>RAPAPATPHAPDHSPAPNSPTLTRPPEGPKFPRVKNWELGSITYDTLCAQSQQDGPCTPRRCLGSLVLPRKLQTRPSPGPPPAEQLLSQARDFINQYYSSIKRSGSQAHEERLQEVEAEVASTGTYHLRESELVFGAKQAWRNAPRCVGRIQWGKLQVFDARDCSSAQEMFTYICNHIKYATNRGNLRSAITVFPQRAPGRGDFRIWNSQLVRYAGYRQQDGSVRGDPANVEITELCIQHGWTPGNGRFDVLPLLLQAPDEAPELFVLPPELVLEVPLEHPTLEWFAALGLRWYALPAVSNMLLEIGGLEFSAAPFSGWYMSTEIGTRNLCDPHRYNILEDVAVCMDLDTRTTSSLWKDKA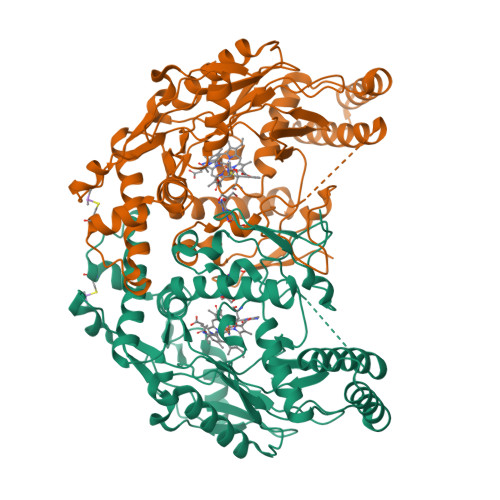AVEINLAVLHSFQLAKVTIVDHHAATVSFMKHLDNEQKARGGCPADWAWIVPPISGSLTPVFHQEMVNYILSPAFRAQPDPW[2x]>MTVGTLVASVLPATVFEDLAYAELYSDPPGLTPLPEEAPLIARSVAKRRNEFITVRHCARIALDQLGVPPAPILKGDKGEPCWPDGMVGSLTHCAGYRGAVVGRRDAVRSVGIDAEPHDVLPNGVLDAISLPAERADMPRTMPAALHWDRILFC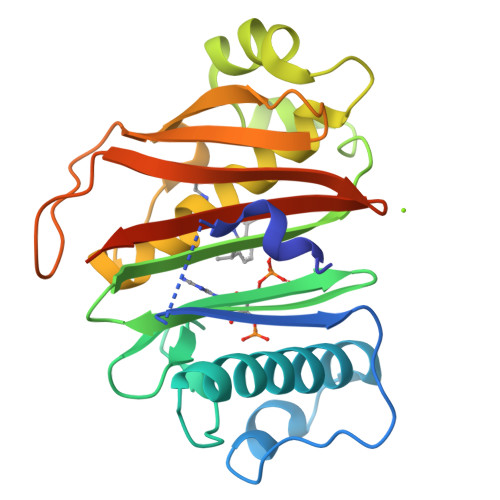AKEATYKAWFPLTKRWLGFEDAHITFETDSTGWTGRFVSRILIDGSTLSGPPLTTLRGRWSVERGLVLTAIVLAGENLYFQSAGHHHHHH[2x]> MRQCVVRRYKMPKNMGVAPRFDTWNEKYEPWEHMKRMGRLVGTGFYIPPEWYNHFRMFPP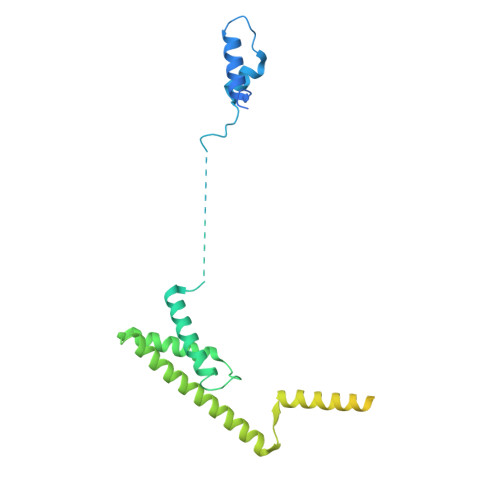INHNFQQEKTLNPHNASEPTQDDTSTLSPERVALRDELARKSRLVASEGMRYYNIFWVRKPLDTMEKEYYELKRRGVDHGEAIRKVLQGFYSGLAVKKRVAAIQAEEAKLTGRFITMREATVVLGVLAKLHKEQLTPHQVSLLAKEQGETTQSGAKLTAIVSRTQPHVNKEASSPATSEAVGSSTEESLSADALASMLSEDGEQSAVGTRYQVEVKETANDSVRQLREKAEDQTGFPDWYTGESPTYSGTS> MKQL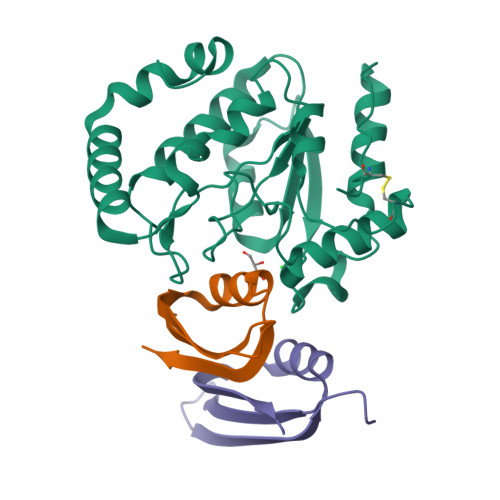LQDSWWNQLKEEFEKPYYQELREMLKREYAEQTIYPDSRDIFNALHYTSYDDVKVVILGQDPYHGPGQAQGLSFSVKPGVKQPPSLKNIFLELQQDIGCSIPNHGSLVSWAKQGVLLLNTVLTVRRGQANSHKGKGWERLTDRIIDVLSERERPVIFILWGRHAQMKKERIDTSKHFIIESTHPSPFSARNGFFGSRPFSRANAYLEKMGEAPIDWCIKDL;>[2x]MVQNDFVDSYDVTMLLQDDDGKQYYEYHKGLSLSDFEVLYGNTADEIIKLRLDKVL>[4x]APAADAAQAHDPLSVQTGSDIPASVHMPTDQQRDYIKREVMVPMRDGVKLYTVIVIPKNARNAPILLTRTPYNAKGRANRVPNALTMREVLPQGDDVFVEGGYIRVFQDIRGKYGSQGDYVMTRPPHGPLNPTKTDETTDAWDTVDWLVHNVPESNGRVGMTGSAYEGFTVVMALLDPHPALKVAAPESPMVDGWMGDDWFHYGAFRQGAFDYFVSQMTAR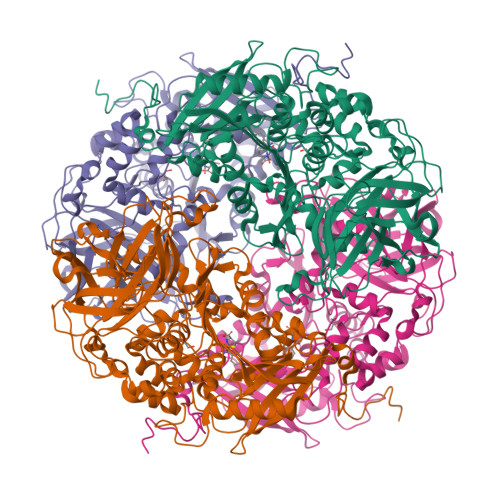GGGNDIPRRDADDYTNFLKAGSAGSFATQAGLDQYPFWQRMHAHPAYDAFWQGQALDKILAQRKPTVPMLWEQGLWDQEDMWGAIHAWQALKDADVKAPNTLVMGPWRHSGVNYNGSTLGPLEFEGDTAHQYRRDVFRPFFDEYLKPGSASVHLPDAIIYNTGDQKWDYYRSWPSVCESNCTGGLTPLYLADGHGLSFTHPAADGADSYVSDPAHPVPFISRPFAFAQSSRWKPWLVQDQREAESRPDVVTYETEVLDEPVRVSGVPVADLFAATSGTDSDWVVKLIDVQPAMTPDDPKMGGYELPVSMDIFRGRYRKDFAKPEALQPDATLHYHFTLPAVNHVFAKGHRIMVQIQSSWFPLYDRNPQKFVPNIFDAKPADYTVATQSIHHGGKEATSILLPVVKQKLGPEQKLISEEDLNSAVDHHHHHH>CKFKFQF[24x]

To address this issue, we have used cryo-electron microscopy (cryo-EM) to determine the molecular structure of an amyloid fibril that is formed from peptide PNF-18. This 7-mer peptide (sequence CKFKFQF) was artificially designed as retroviral transduction enhancer and increases HIV-1 infection rates of TZM-bl cells by a factor of more than a hundred-fold. Each protofilament (PF) is built by two paired cross-β sheets that interact by the hydrophobic side of the amphipathic peptide, while the polar residues are pointing outwards, creating a positive surface. These structural features provide insights into the molecular basis of amyloid polymorphism and virus binding, and improves our understanding of the molecular basis of peptide nanofibrils as retroviral transduction enhancers.

We achieved a spatial resolution of 2.86 Å, based on the 0.143 Fourier shell correlation (FSC) criterion. There were, depending on the position of the peptide stack in the fibril structure, three topological types of peptide stacks (α, β and γ) that were arranged into pairs, which we refer to hereafter as PFs. Morphology II consists of three PFs, two peripheral ones and a central one, and six peptides in each molecular layer. The peptide conformation is kinked and shows two chemically different sides: a hydrophobic side that is formed by residues Phe3, Phe5, and Phe7 and a polar one that is formed by the side chains of Cys1, Lys2, Lys4, Gln6 as well as the N- and C-terminal groups of the polypeptide backbone. The peptide’s amphipathic properties lead to two modes by which two peptides (or cross-β sheets) may interact within the plane of the fibril cross-section: a hydrophobic and a polar contact mode. The hydrophobic contact mode occurs between the two type α peptide stacks and between a type β and a type γ stack. The polar contact mode, which occurs between type α and β peptide stacks, involves an interdigitation of the side chains of residues Lys4 and Gln6, similar to a steric zipper. The zipper-like region is flanked on both sides by an intermolecular charge pair that is formed by the ε-amino group of Lys4 and α-carboxy group of the peptide C-terminus. Only the peptides in stack γ, which are bound through the hydrophobic contact mode to stack β, adopt an angle of almost 45° relative to the fibril z-axis. Morphology II shows a strongly cationic Coulomb surface potential, which originates mainly from the side chains of Lys2 and Lys4, and the α-amino group of Cys1.Muramidases are N-acetylmuramide glycanhydrolases which cleave the β-1,4-glycosidic bond between N-acetylmuramic acid (NAM) and N-acetylglucosamine (NAG) in the carbohydrate backbone of the bacterial cell-wall peptidoglycan. Here, the identification, characterization and X-ray structure of a novel fungal GH24 muramidase from Trichophaea saccata is first described, in which an SH3-like cell-wall-binding domain (CWBD) was identified by structure comparison in addition to its catalytic domain. A ‘domain-walking’ approach, searching for other sequences with a domain of unknown function appended to the CWBD, was then used to identify a group of fungal muramidases that also contain homologous SH3-like cell-wall-binding modules, the catalytic domains of which define a new GH family. The properties of some representative members of this family are described as well as X-ray structures of the independent catalytic and SH3-like domains of the Kionochaeta sp., Thermothielavioides terrestris and Penicillium virgatum enzymes.

The natural enzyme from Kionochaeta sp. lacks the CWBD and we describe its crystal structure. There is one subunit in the asymmetric unit, with two cadmiums, one with full occupancy, coordinated by His29 and His67 from the symmetry-related molecule and by four waters, and a second with an occupancy of 0.23, coordinated by His60 and five waters. There were no close sequence homologues with known X-ray structures for this enzyme. Similar to that of gp13, the Kionochaeta GH184 domain is mostly an α-helix bundle (CATH; Sillitoe et al., 2021). It can be roughly divided into two subdomains, with one subdomain all α-helical and the second, residues 42–88, containing two (or four in TtGH184 described below) short β-strands and two very short α-helices with connecting loops. There are three poorly ordered ethylene glycol molecules from the cryoprotectant in the KsGH184 structure, two of which are close to the active site. A mutational study confirmed that Glu41 is essential for catalysis. Glu41 corresponds to the suggested catalytic Glu45 in gp13 and is located in the all-α subdomain at the end of helix 2.

> LVLPGLDALQTRNALAIIAEAKKENVGPHGCQAAITTGLTESSLRILANNAVPPSLQYPHDGLGSDHDSIGIFQQRASIYKDIRCDMDAACSASQFFKVMKGVSGWQTLDVATLCQRVQKSAYPAAYQKFTALAVGVCKAGGL>[4x]MKIVLVLYDAGKHAADEEKLYGCTENKLGIANWLKDQGHELITTSDKEGGNSVLDQHIPDADIIITTPFHPAYITKERIDKAKKLKLVVVAGVGSDHIDLDYINQTGKKISVLEVTGSNVVSVAEHVLMTMLV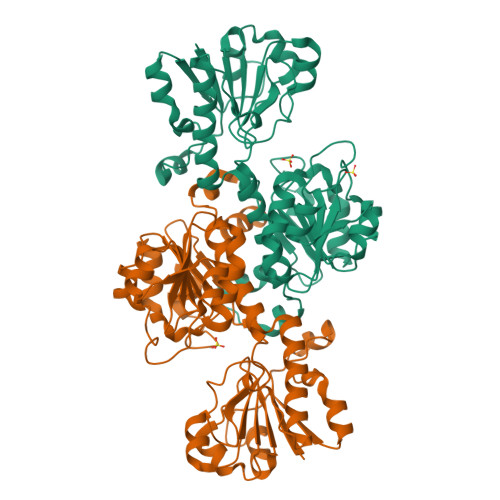LVRNFVPAHEQIINHDWEVAAIAKDAYDIEGKTIATIGAGRIGYRVLERLVPFNPKELLYYDYQALPKDAEEKVGARRVENIEELVAQADIVTINAPLHAGTKGLINKELLSKFKKGAWLVNTARGAICVAEDVAAALESGQLRGYGGDVWFPQPAPKDHPWRDMRNKYGAGNAMTPHYSGTTLDAQTRYAEGTKNILESFFTGKFDYRPQDIILLNGEYITKAYGKHDKK> MANQRMLGFVHTAQRMPDKRPAAERRQDFAEIYARFSDERANEQANRCSQCGVPFCQVHCPVSNNIPDWLKLTSEGRLEEAYEVSQATNNFPEICGRICPQDRLCEGNCVIEQSTHGAVTIGSVEKYINDTAWDQGWVKPRTPSRELGLSVGVIGAGPAGLAAAEELRAKGYEVHVYDRYDRMGGLLVYGIPGFKLEKSVVERRVKLLADAGVIYHPNFEVGRDASLPELRRKHVAVLVATGVYKARDIKAPGSGLGNIVAALDYLTTSNKVSLGDTVEAYENGSL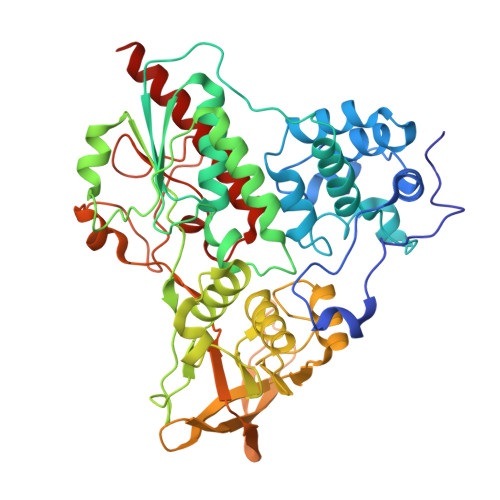NAAGKHVVVLGGGDTAMDCVRTAIRQGATSVKCLYRRDRKNMPGSQREVAHAEEEGVEFIWQAAPEGFTGDTVVTGVRAVRIHLGVADATGRQTPQVIEGSEFTVQADLVIKALGFEPEDLPNAFDEPELKVTRWGTLLVDHRTKMTNMDGVFAAGDIVRGASLVVWAIRDGRDAAEGIHAYAKAKAEAPVAVAAE> MTAEPATKKIKLELSDPSEPLTQSDVIAFQKEALFRCINRRRVDFEALRKQYELSRRECIDVS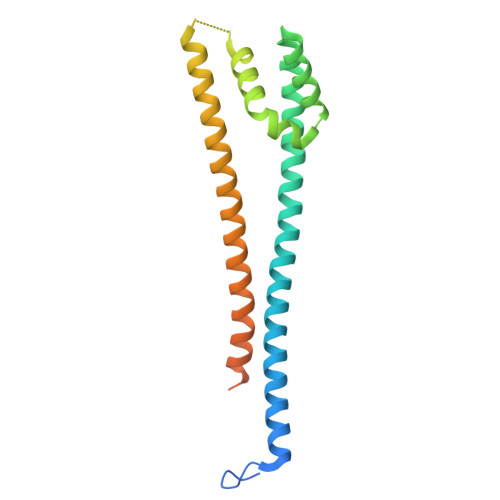RKLANIMALIVTLARFIETFCTDANEKQLCREIAQGDETLIVQRSDSFMKLLTKYGKPNTTDSNTNSNASDHIQELTTELKNLRKSKEELFYENSQLTEEISALKEYYTNIIRKYDRDESFTIKRVFKEDKTDAVKELREDEKESNENN triphenylphosphane | C18 H15 P | 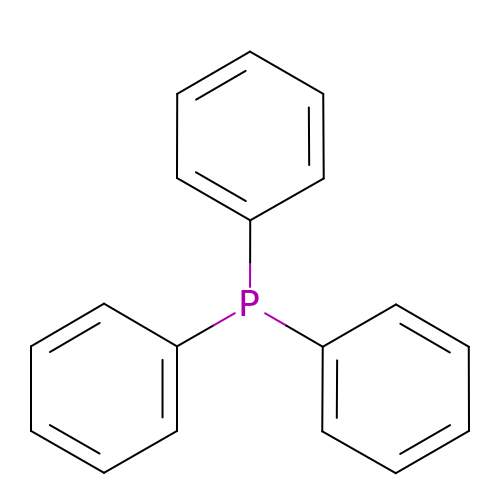RIOQSEWOXXDEQQ-UHFFFAOYSA-N>[2x]MSFSSKPTVLASRVESDSAINVMKWKTVSTIFLVVVLYLIIGATVFKALEQPQEISQRTTIVIQREKFLRAHPCVSDQELDELIQQIVAADNAGIIPLGAS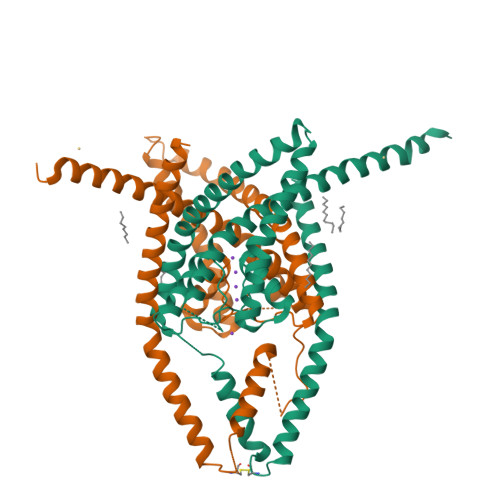SNQVSHWDLGSSFFFAGTVITTIGFGNISPRTEGGKIFCIIYALLGIPLFGFLLAGVGDQLGTIFGKGIAKVEDTFIKWNVSQTKIRIISTIIFILFGCVLFVALPAVIFKHIEGWSALDAIYFVVITLTTIGFGDYVAGGSDIEYLDFYKPVVWFWILVGLAYFAAVLSMIGDWLRVIAKKTKEAVGEFRAHAAEWTANVTSNSLEVLFQ>[2x]GAAUUGCGGGAAAGGGGUCAACUUCCGUUCAGUACCAAGUCUCAGGGGAAACUUUGAGAUGGCCUUGCAAAG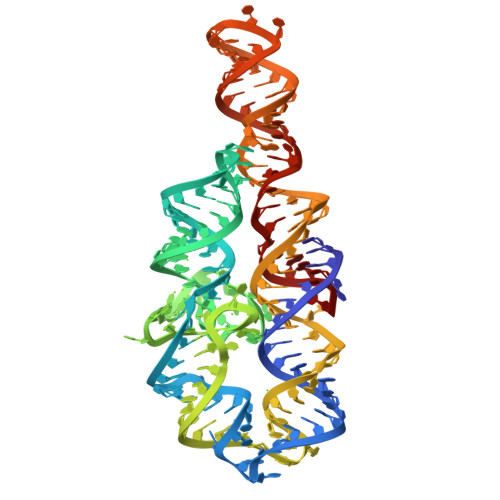GGUAUGGUAAUAAGCUGACGGACAUGGUCCUAACCACGCAGCCAAGUCCUAAGUCAACAGAUCUUCUGUUGAUAUGGAUGCAGUUCA>MKDIAIRGYCDRPSVATGETIRFYVSANETRGTFDAELVRLIHGDSNPAGPGYKEEAIKSDLEGQYPARFQRTQFGSYVEVADPDAGLQPDGAFSVHLFLWSTTPSRGRQGIASRWNDERQSGWNLAIEDGRVVFTIGDGSGATSSVVSDRPLFQQIWYSITGVYDPEKKQLRLYQKSVVNRTNSRFGLVVPLDSDCAVSADATVKAADSETSLLIAGLGEAAAQDGRTWCIAHYNGKVDAPKIYGCALGQDDAEKLSRGEIVRPISRLAHWDFSAGIGLNGIPTDHVVDASGYGHHGRCMNQPSRGSTGWNWDGHEENFIHCPEQYGALWFHEDCLDDCRWEKDFEFTVPEGLKSDFYAVKIRYEDTEDYIPFFVLPPRGTATAPILVIASTLSYLAYANEQIMHKADIGQAVAGHTPVLNEND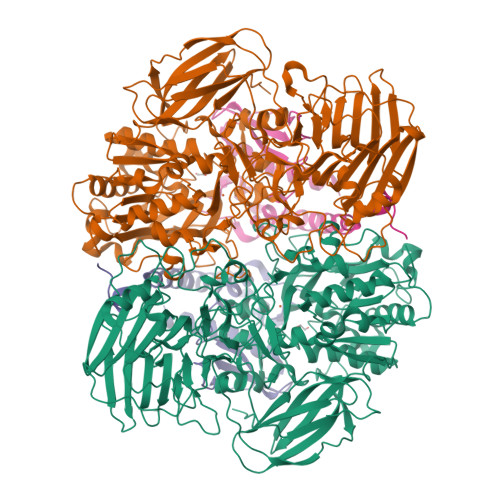VELHKNLSYYGLSTYDGHIDGRGVQYTSWRRPIMNLRPKHRQGFGSIWELPADLHLIDWLNHNGFEYDVATEHDLNDQGAELLRRYKVVLTGSHPEYQTWANADAWEDYLADGGRGMYLAANGMYWIVEVHPEKPWVMEVRKELGVTAWEAPPGEYHYSTNGRRGGRFRGRARATQKIWGTGMSSFGFDHSGYFVQMPDSQDERVAWIMEGIDPEERIGDGGLVGGGAGGYELDRYDLALGTPPNTLLLASSVEHSVVYTVIPDDKAFPHPGMNGGEHPFVRADITYFSTANGGGMFATSSISWLGSLSWNDYDNNVSKMTKNVLNQFIKDEPAPRVKLAAALEHHHHHH[8x];>MTEASESCVRDPSNYRDRSADWYAFYDERRRKEIIDIIDEHPEIVEEHAANPFGYRKHPSPYLQRVHNYFRMQPTFGRYYIYSEREWDAYRIATIREFGELPELGDERFKTEEEAMHAVFLRRIEDVRAELA[8x]> EASIPTVERSTRMSNPWKAFMEKYDIERTHSSGVRVDLGEDAEVENAKYRIPAGRCPVFGKGIVIENSDVSFLRPVATGDEKLKDGGFAFPNANDHISPMTLANLKERYKDNVEMMKLNDIALCRTHAASFVMAGDQNSNYRHPAVYDEKEKTCHMLYLSAQENMGPRYCSPDAQNRDAVFCFKPDKDESFENLVYLSKNVRNDWDKKCPRKNLGNAKFGLWVDGNCEEIPYVKEVEAEDLRECNRIVFGASASDQPTQYEEEMTDYQKIQQGFRQNNREMIKSAFLPVGAFNSDNFKSKGRGFNWANFDSVKKKCYIFNTKPTCLINDKNFIATTALSHPQEVDLEFPCSIYKDEIEREIKKQSRNMNLYSVDGERIVLPRIFISNDKESIKCPCEPERISQSTCNFYVCNCVEKRAEIKENNQVVIKEEFRDYYENGEEKSNKQMLLLEQKLISEEDLNSAVDHHHHHH;> MDISQHATDIGMGPATSCYTSTIPPPKQVCIQQAVKATL

Two of these, Apical Membrane Antigen 1 (AMA1) and the Rhoptry Neck (RON) complex comprising RON2, RON4 and RON5, play a crucial role at the MJ.. In this invasion model, AMA1 and the RON complex then bind together linking the merozoite and erythrocyte membranes to form an essential structural component that maintains the MJ ring. The receptor-binding site on P. falciparum and T. gondii AMA1 (PfAMA1 and TgAMA1, respectively) comprises a region on Domain 1 of the ectoplasmic domain termed the hydrophobic groove and a region immediately adjacent that becomes exposed when the mobile Domain 2 (D2) loop (residues Ser347-His393) is displaced by the incoming ligand. We have determined the crystal structure of AMA1 from P. vivax (PvAMA1) in complex with a 39-residue peptide corresponding to the extracellular region of RON2 from P. vivax (PvRON2sp1) and, in addition, the structure of the cross-reaction complex formed between PvRON2sp1 and PfAMA1.

Crystals were obtained for complexes formed between PvAMA1 strain Sal-1 (comprising domains D1, D2 and D3), or PfAMA1 strain FVO (comprising domains D1 and D2), and the peptide PvRON2sp1 (39 residues: Met2034 to Leu2072; PvRON2 residue numbering from PlasmoDB entry PVX_117880). A total of 33 of the 39 residues of the bound PvRON2sp1 ligand could be followed in the electron density from Ser2037 to Lys2069. The PvRON2sp1 peptide occupies a groove of PvAMA1 that is located mostly on domain D1 and contributes the majority of the contacts; however, loop regions surrounding the groove also contribute to the binding. The peptide is boomerang-shaped with one wing formed by a disulphide-bridged β-hairpin loop comprising the central segment of the peptide between residues Cys2051 to Cys2063, while the other wing is formed by the flanking N- and C-terminal segments. The solvent-inaccessible surface at the PvAMA1-PvRON2sp1 buried at interface is 2893 Å2. The loop 129–134 undergoes a significant conformational change upon binding PvRON2sp1, with Asp133 moving by more than 6 Å, and the loop 171–176, which is completely disordered in the apo PvAMA1, makes contacts with PvRON2sp1 and could be completely traced in the electron density of the complex. The loop 148–151 also contacts the peptide ligand but shows no important structural differences with respect to that of the free PvAMA1. Finally, residues 296 and 297 at the N-terminal base of the disordered D2 loop contact PvRON2sp1. Although this pocket is absent in the PvAMA1 crystal structure, the smaller side chain of the equivalent PvRON2 residue, Thr2055, is accommodated within the flatter topology of this region of the binding site but is positioned further out relative to Arg2041 in the PfAMA1-PfRON2sp1 homocomplex and, indeed, to Thr2055 in the P. falciparum heterocomplex. By contrast, the side chain of PvAMA1-Arg180, the residue equivalent to PfAMA1-Lys235, is constrained closer to the protein surface by contacts with a symmetry-related molecule, closing off the pocket.FtsEX, an important component of the divisome, is mainly recognized for its involvement in activating the degradation of sPG through amidases via the periplasmic factor EnvC. FtsEX belongs to the Type VII ABC superfamily, which includes LolCDE and MacB. In contrast to the reported ABC transporters, FtsEX neither transports anything across the membrane nor extracts substances from the membrane but interacts with EnvC to form the sPG hydrolysis machinery to separate the daughter cells during cell division. The activation of AmiA and AmiB by EnvC is controlled by the cell division protein complex FtsEX, which induces conformational changes in EnvC through ATP hydrolysis.

In this study, we constructed the FtsEE163Q mutant, which was expected to abolish ATPase activity but retain ATP-binding ability. FtsEE163QX was successfully expressed and purified in the presence of ATP, while the sPG hydrolysis machinery complex FtsEE163QX-EnvC with ATP was further obtained by in vitro reconstitution. We then determined the cryo-EM structure of ATP-bound E. coli FtsEE163QX and ATP-bound FtsEE163QX-EnvC at overall resolutions of 3.05 Å and 3.11 Å, respectively, using the gold standard Fourier shell correlation based on the 0.143 criterion. For FtsEX cryo-EM map, we built a model including FtsE, FtsX (without the periplasmic domain). The FtsEX complex structure shows a severely disordered periplasmic structure, indicating that this domain is highly flexible. Notably, the cryo-EM map of the FtsX periplasmic domain in FtsEE163QX-EnvC is significantly clearer than that of FtsEE163QX. This suggests that the periplasmic domains of FtsX can be stabled when bound with EnvC, which helped in resolving the cryo-EM map of these regions. Our results revealed that a single FtsX molecule exhibits a topological structure comprising 4 transmembrane helices (TMs) named TM1-TM4. Between TM2 and TM3, there is a helix α3 corresponding to the coupling helix. The interaction between FtsE and FtsX primarily occur through the coupling helix, a fundamental component of ABC transporters that links the NBD and TMD to drive conformational changes in the TMD and other subunits upon ATP consumption.

>[2x]MIRFEHVSKAYLGGRQALQGVTFHMQPGEMAFLTGHSGAGKSTLLKLICGIERPSAGKIWFSGHDITRLKNREVPFLRRQIGMIFQDHHLLMDRTVYDNVAIPLIIAGASGDDIRRRVSAALDKVGLLDKAKNFPIQLSGGEQQRVGIARAVVNKPAVLLADQPTGNLDDALSEGILRLFEEFNRVGVTVLMATHDINLISRRSYRMLTLSDGHLHGGVGHE;>[2x]MNKRDAINHIRQFGGRLDRFRKSVGGSGDGGRNAPKRAKSSPKPVNRKTNVFNEQVRYAFHGALQDLKSKPFATFLTVMVIAISLTLPSVCYMVYKNVNQAATQYYPSPQITVYLQKTLDDDAAAGVVAQLQAEQGVEKVNYLSREDALGEFRNWSGFGGALDMLEENPLPAVAVVIPKLDFQGTESLNTLRDRITQINGIDEVRMDDSWFARLAALTGLVGRVSAMIGVLMVAAVFLVIGNSVRLSIFARRDSINVQKLIGATDGFILRPFLYGGALLGFSGALLSLILSEILVLRLSSAVAEVAQVFGTKFDINGLSFDECLLLLLVCSMIGWVAAWLATVQHLRHFTPE> GPGSDRPPPYVAPPSYEG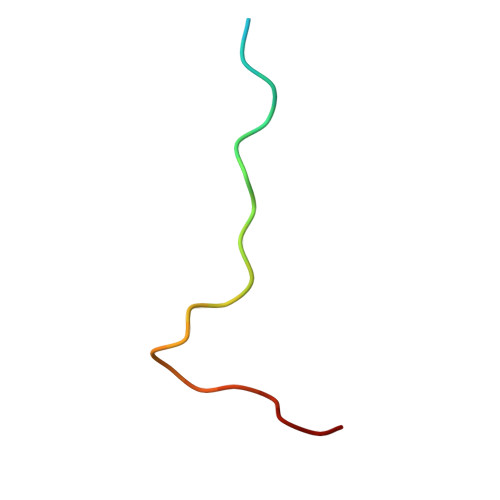PHRTLG>[4x]STAFTGVRDVPAQQIVNEMKVGWNL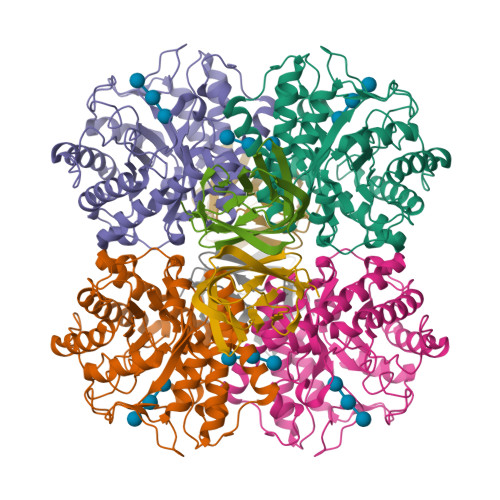GNTMDAIGGETNWGNPMTTHAMINKIKEAGFNTLRLPVTWDGHMGAAPEYTIDQTWMKRVEEIANYAFDNDMYVIINLHHENEWLKPFYANEAQVKAQLTKVWTQIANNFKKYGDHLIFETMNEPRPVGASLQWTGGSYENREVVNRYNLTAVNAIRATGGNNATRYIMVPTLAASAMSTTINDLVIPNNDSKVIVSLHMYSPYFFAMDINGTSSWGSDYDKSSLDSEFDAVYNKFVKNGRAVVIGEMGSINKNNTAARVTHAEYYAKSAKARGLTPIWWDNGYSVAGKAETFGIFNRSNLTWDAPEVMKAFIKGIGGSS;>SAVEVTYAITNSWGSGASVNVTIKNNGTTPINGWTLKWTMPINQTITNMWSASFVASGTTLSVTNAGYNGTIAANGGTQSFGFNINYSGVLSKPTGFTVNGTECTVK[4x]>MARKYFVAANWKCNGTLESIKSLTNSFNNLDFDPSKLDVVVFPVSVHYDHTRKLLQSKFSTGIQNVSKFGNGSYTGEVSAEIAKDLNIEYVIIGHHERRKYFHETDEDVREKLQASLKNNLKAVVCFGESLEQREQNKTIEVITKQVKAFVDLIDNFDNVILVYEPLWAIGTGKTATPEQAQLVHKEIRKIVKDTCGEKQANQIRILYGGSVNTENCSSLIQQEDIDGFLVGNASLKES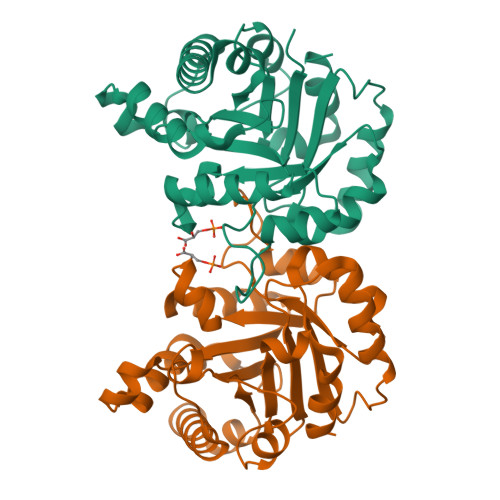FVDIIKSAM[4x]> DPGCLPDWSSYKGHCYKVFKKVGTWEDAEKFCVENSGHLASIDSKEEADFVTKLASQTLTKFVYDAWIGLRDESKTQQCSPQWTDGSSVVYENVDEPTKCFGLDVHTEYRTWTDLPCGEKNPFICKSRLPH;> DEGCLPDWSSYKGHCYKVFKVEKTWADAEKFCKELVNGGHLMSVNSREEGEFISKLALEKMRIVLVWIGLSHFWRICPLRWT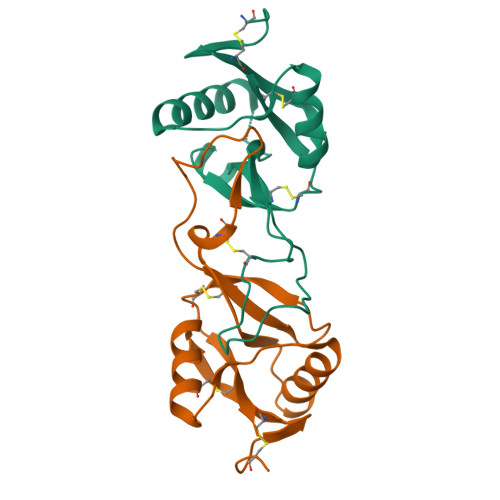DGARLDYRALSDEPICFVAESFHNKWIQWTCNRKKSFVCKYRV8-cyclohexyl-N-methoxy-5-oxo-2-{[4-(2-pyrrolidin-1-ylethyl)phenyl]amino}-5,8-dihydropyrido[2,3-d]pyrimidine-6-carboxamide | C27 H34 N6 O3 | 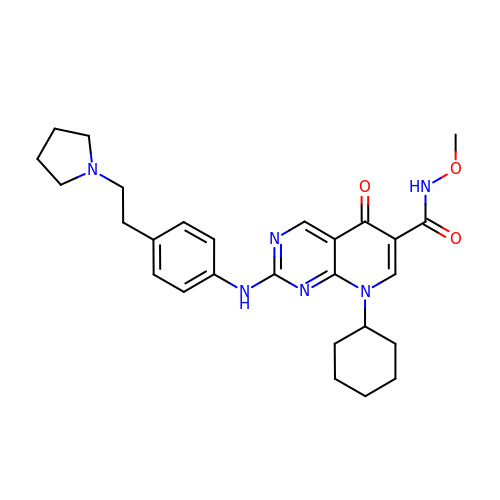LYINTIKJROJCGF-UHFFFAOYSA-N>[4x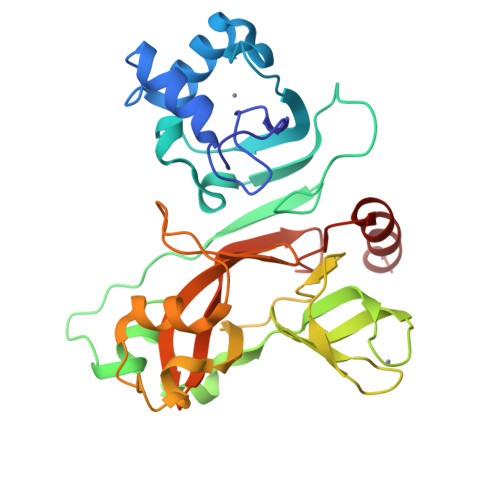]SMAYTRYVDNNFCGPDGYPLECIKDLLARAGKASCTLSEQLDFIDTKRGVYCCREHEHEIAWYTERSEKSYELQTPFEIKLAKKFDTFNGECPNFVFPLNSIIKTIQPRVEKKKLDGFMGRIRSVYPVASPNECNQMCLSTLMKCDHCGETSWQTGDFVKATCEFCGTENLTKEGATTCGYLPQNAVVKIYCPACHNSEVGPEHSLAEYHNESGLKTILRKGGRTIAFGGCVFSYVGCHNKCAYWVPRASANIGCNHTGVVGEGSEGLNDNLLEILQK> ESQPDPMPDDLHKSSEFTGTMGNMKYLYDDHYVSATKVKSVDKFL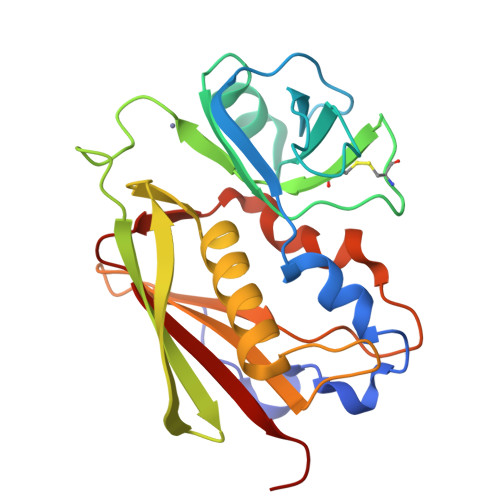AHDLIYNISDKKLKNYDKVKTELLNEDLAKKYKDEVVDVYGSNYYVNCYFSSKDNKWWHGKTCMYGGITKHEGNHFDNGNLQNVLVRVYENKRNTISFEVQTDKKSVTAQELDIKARNFLINKKNLYEFNSSPYETGYIKFIENNGNTFWYDMMPAPGDKFDQSKYLMMYNDNKTVDSKSVKIEVHLTTKNG>MKIVDVLCTPGLTGFYFDDQRAIKKGAGHDGFTYTGSTVTEGFTQVRQKGESISVLLVLEDGQVAHGDCAAVQYSGAGGRDPLFLAKDFIPVIEKEIAPKLIGREITNFKPMAEEFDKMTVNGNRLHTAIRYGITQAILDAVAKTRKVTMAEVIRDEYNPGAEINAVPVFAQSGDDRYDNVDKMIIKEADVLPHALINNVEEKLGLKGEKLLEYVKWLRDRIIKLRVREDYAPIFHIDVYGTIGAAFDVDIKAMADYIQTLAEAAKPFHLRIEGPMDVEDRQKQMEAMRDLRAELDGRGVDAELVADEWCNTVEDVKFFTDNKAGHMVQIKTPDLGGVNNIADAIMYCKANGMGAYCGGTCNETNRSAEVTTNIGMACGARQVAAKPGMGVDEGMMIVKNEMNRVLALVGRRKKLGPEQKLISE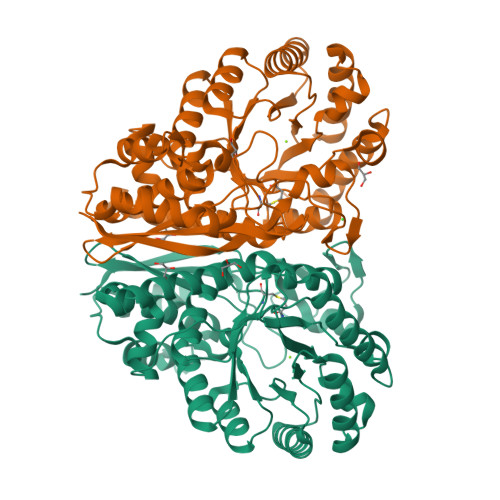EDLNSAVDHHHHHH[2x]> EENFNADHPFIFFIRHNPSANILFLGRFS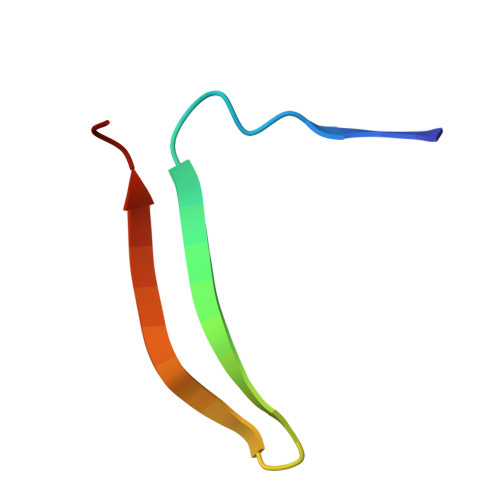SP>QQVCTTQAETHPALSWSKCTSGGSCTTQAGKVVLDANWRWTHAYPSGNNCYNGNTWDATLCPDDATCAKNCCLEGADYSGTYGVTTSGNQLTIDFVTQSANKNVGARLYLMASDTAYEEFTLLNNEFSFDVDVSALPCGLNGALYFVSMDADGGASKYPTNLAGAKYGTGYCDSQCPRDLKFISGQANVEGWQPSSNNANTGIGGHGSCCSEMDIWEANSISQALTPHPCETVGQVTCSGDDCGGTYSNNRYGGTCDPDGCDWNPYRLGNHTFYGPGSGFTVDTTKKITVVTQFSSTGINRYYVQNGVKFVQPNASGLSGYTGNTINSAYCSAEQTAFGGTSFTDKGGLTQMNKALSGGMVLVLSLWDDYAANMLWLDSTYPTNDTASTPGAARGTCSTSSGVPATVEQQSPNSKVVFSNIKFGPIGSTG[2x]

In many of these fungi, the major secreted enzymes are glycoside hydrolase family 7 (GH7) cellobiohydrolases (CBH). CBHs within GH7 are readily distinguished because several loops are further elongated, effectively enclosing the active site in a tunnel. This enables the CBHs to act processively along a cellulose chain and cleave off numerous cellobiose units before detachment from the substrate, which is believed to be key to their efficiency on highly crystalline cellulose. The GH7 CBHs of T. harzianum (ThaCel7A) and T. atroviride (TatCel7A) share the GH7_CD-linker-CBM1 bimodular organization and are very similar to each other and to TreCel7A, with ~ 80% pairwise sequence identities.

The TatCel7A_CD protein was successfully crystallized, and two structures were solved, one apo structure without sugars bound (APO) and one thio-cellotrioside complex (SG3). Both structures were refined at 1.7 Å resolution in space group P21 with two protein chains, A and B, in the asymmetric unit. In the SG3 structure, from co-crystallization with thio-linked cellotriose, there are two cellotrioside molecules bound to each protein chain, in subsites − 6/− 5/− 4 and + 1/+ 2/+ 3, respectively. For the ligand in the − 6/− 5/− 4 position at the tunnel entrance, all glucose residues adopt the 4C1 chair conformation, but the C1 hydroxyl at the reducing end in subsite − 4 is predominantly in the α-position, with very weak density for a β-hydroxyl. Interestingly, the sugar ring at each site is flipped upside down compared to the orientation in the Michaelis complex of TreCel7A. The binding may represent a sliding intermediate during processive cellulose hydrolysis. The other thio-cellotrioside molecule in the SG3 structure, at + 1/+ 2/+ 3, is in register and aligns well with the glycan binding at the product sites of the TreCel7A Michaelis complex. The + 1 and + 2 glucosides are in 4C1 chair conformations, whereas the + 3 unit at the reducing end adopts a 1S3 skew conformation, again with α-hydroxyl predominance at the anomeric carbon. Overall, the TatCel7A_CD structures are very similar (0.18 Å root mean square deviation, RMSD), although there is a general ‘tightening’ of the protein around the active site in SG3 compared to APO, which is most pronounced at the A4-loop near the product sites.N-(4-AMINOBUTANOYL)-S-(4-METHOXYBENZYL)-L-CYSTEINYLGLYCINE | C17 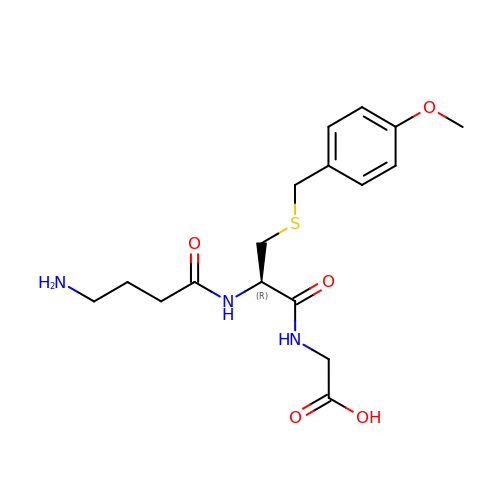H25 N3 O5 S | OMOPDEZZBQHMGS-AWEZNQCLSA-N> GCCCGGAUAGCUCAGUCGGUAGAGCAGCGGUAAAACAGCCUGUGGG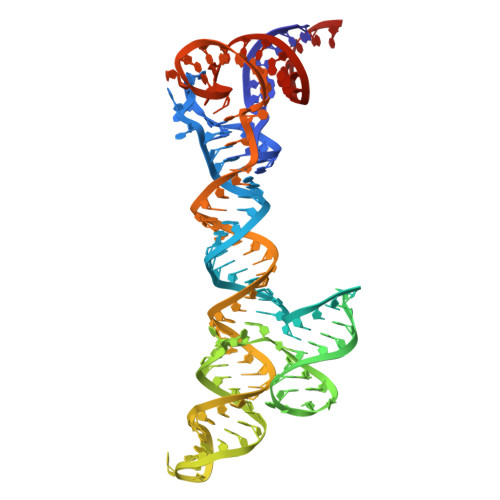UUGAUCCCACCCACAGGGCCCAUUGGGCGCUAGCACUCUGGUAUCACGGUACCUUUGUGCGCCUGUUUUACCGCGGGUCCAGGGUUCAAGUCCCUGUUCGGGCGCCA>[2x]GPGPSRPSASWQNSVSERPPYSYMAMIQFAINSTERKRMTLKDIYTWIEDHFPYFKHIAKPGWKNSIRHNLSLHDMFVRETSANGKVSFW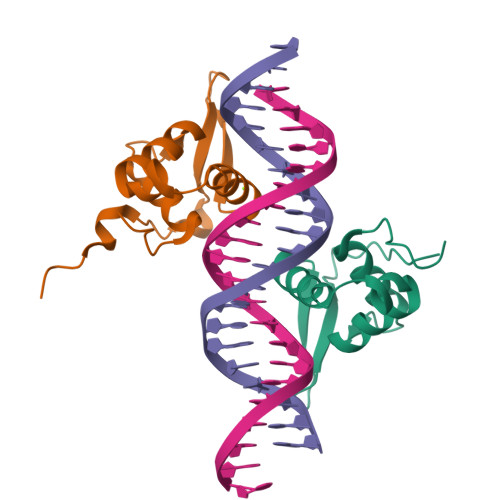TIHPSANRYLTLDQVFKPLDPGSPQLPEHLESQQKRPNPELRRNMTIKTELP> GGLVPRGSHMFIMIGERINGMFKDIREAILNKDPRPIQEWARRQAEKGAHYLDVNTGPTADDPVRVMEWLVKTIQEVVDLPCCLDSTNPDAIEAGLKVHRGHAMINSTSADQWKMDIFFPMAKKYEAAIIGLTMNEKGVPKDANDRSQLAMELVANADAHGIPMTELYIDPL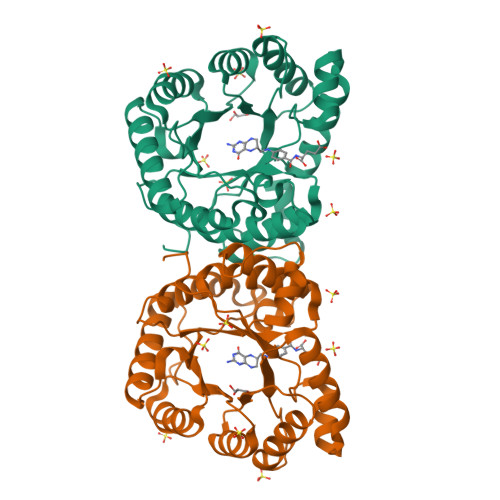ILPVNVAQEHAVEVLETIRQIKLMANPAPRTVLGLSNVSQKCPDRPLINRTYLVMAMTAGLDAAIMDVDDDALVDAAATAHILLNKEIYCDSYLKTFRQK> ADSDSVLKTVIYSSSGALFMGVWNPSSSGYSDTYSRRIADLVFDSGIPYGIDGVPHPYHCHVVDYKSDVTVPEDAVIFNSTTDTWVAAHAGETAKTYARIECDRPYFHDGHKLSAADVMYSLAWSWEWTTQDGDDDPYYDASEADWSGEYMNTILGIKLVEQTDDRMVFDVYHNHYFPASEIMTAAYVVPFTGTPWQLWYAMSELVAHNPKYSWSESSEDVEQLDQINPSHAQAIKEKLLELKQSKPIPEFLKPYIEDENAATAAYDSIAKFMDEHNHAVIGQGPYYVDEYQPENLFVRIKKFDKWTIPAFAEPEYQVDPYYKTIEVYGIQNEDTAILEVANGHYDILWYPFAAYRFTGLSDEQRANIKLYRSTSAFGDIVWNPVHDQDNPYVITVGDKKYFNPFAVRKVRFAIQYMVNRAYITQNIFQGSAGPMFTPWTSTETGFEYVRPVVDAFGLTEQSDEDLAMKLFEEGMQEAAQELAKMGYELKKGDDGKWYFNGEPVKVVGLGRVEDERKDVATYIVEEVMKKLGFDAEAKIVDRRTASGTVYTSDPSSYQWNFYTEGWVSSSNVKFSTTRII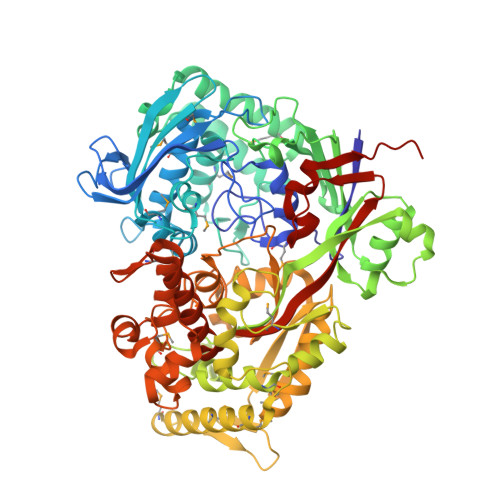QYYSSYWYAPGLVGWKWTPENTQRVTMEEVLKFLGNGDIQAGLDSLGLSYYNTVDKIQPLLNWTADDFALVIYSGEANGVKMDSEDKYWDFNRLGTAIGIYEGYRTFLYENWEFYAASKDIEIKLVDPVAGLASDWAIRSARPVVEHHHHHH Upon complement activation, a cascade of proteolytic events generates the complement effectors, including the anaphylatoxins C3a and C5a. Anaphylatoxin signalling through the G-protein coupled receptors (GPCRs) C3aR and C5aR leads to various cellular responses including chemotaxis, oxidative burst, the release of pro-inflammatory molecules and activation of the adaptive immune system. As for C3a, C5a activity is regulated by carboxypeptidases that cleave off the C-terminal arginine residue, producing the C5a-desArg molecule which has a distinct bioactivity pattern and generally a much lower potency than C5a, in part owing to its tenfold to 100-fold decrease in C5aR binding affinity. Here, we have reported the crystal structures of the human C5aR antagonist hC5a-A8 and of the two murine anaphylatoxins mC5a and mC5a-desArg.

To assess whether this property was specific to the human C5a proteins or whether this is a general feature of C5a, we also determined the structures of mouse C5a and C5a-desArg (mC5a and mC5a-desArg) at 1.4 and 2.1 Å resolution, respectively. Both murine proteins fold into a four-helix bundle motif as observed for hC5a. mC5a and mC5a-desArg crystals both displayed P43 symmetry with very similar unit-cell parameters and diffracted to 1.4 and 2.1 Å resolution, respectively. In both structures, the atomic model was traced between residues Asn679 and Ser746, which corresponds to the four-helix bundle core, with helix H1 extending between Asn679 and Tyr694, helix H2 formed by residues Ser697–Arg708, helix H3 encompassing residues Thr714–Val722 and helix H4 comprising residues Gly725–Ser746. The overall fold is also stabilized by three disulfide bridges in both mC5a and mC5a-desArg: Cys702–Cys728 (H2–H4), Cys703–Cys735 (H2–H4) and Cys715–Cys736 (H3–H4). The C-terminus of mC5a and mC5a-desArg (region Pro747–Arg755/Gly754) was not visible in the electron density, again suggesting its high flexibility. Surprisingly, a blob of density that assumed the shape of an arginine was visible in the mC5a structure. This density is observed in the groove between the helix H1 N-terminus and the helix H2 C-terminus of monomer A in the asymmetric unit and is located within hydrogen-bonding distance of Arg743 of the same monomer. Inspection of the crystal packing reveals that this density could represent the C-terminal Arg755 of mC5a from a neighbouring symmetry-related molecule, in which the Cα atom of the last modelled residue, Glu745, is separated by 21 Å from the putative position of this Arg755 Cα atom, a distance that could accommodate a stretch of nine residues assuming a random-coil nonlinear conformation. As expected, mC5a is a full agonist of mC5aR and can activate the receptor with an EC50 of 0.57 ± 0.13 nM.

>[4x]GANLHLLRQKIEEQAAKYKHSVPKKCCYDGARVNFYETCEERVARVTIGPLCIRAFNECCTIANKIRKESPHKPVQLGR>KNLRDLEPGIHTDLEGRLTYGGYLRLDQLLSAQQPLSEPAHHDEMLFIIQSQTSELWLKLLAHELRAAIVHLQRDEVWQCRKVLARSKQVLRQLTEQWSVLETLTPSEYMGFRDVLGPSSGFQSLQYRYIEFLLGNKNPQMLQVFAYDPAGQARLREVLEAPSLYEEFLRYLARFGHAIPQQYQARDWTAAHVADDTLRPVFERIYENTDRYWREYSLCEDLVDVETQFQLWRFRHMRTVMRVIGFKRGTGGSSGVGFLQQALALTFFPELFDVRT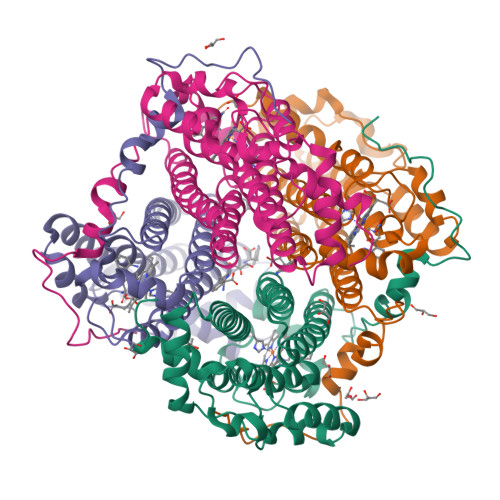SVGVDN[8x]>MYRYEKKGPKRGVALYSYSAEFGLTKTLEDCFEDLHDMGAHGIEILANTHIENYPYPTDEWVEKWWRLCDKYEIVPVEYGNWIDSHVLGDRDLTTEESVEMLKRDIRLAHRLGFTVMRTKMPVINDLLEPVENWKEIIKGALPLAEELGIKMCPEIHTPSNLKGKLVNDFVEFIKETGTKNFGLNIDFSVFRTSFAEGEWVDPNYTPNKPEDIIPLLPYVYCCHAKFIHMSDDFKETTIPYEEVVKTMEDNGYEGYLLSEYEGADKYDEGYEVGQTLRKHHILLKNLLGD[4x];>MEKQVIQSVGFRNIKNGNGEITGFQFKVKLPYYRGVFLSQIRPGTLFVDGQKIEKDQITWTINGEEYTNQEMRGDFKTHWATTKPAVLKVKMPGGLAQGYHDLKYGFCFTSSYMPPIIQDGLDPDKESMVYMPEFGHHVNERRLLIVKLAAALEHHHHHH[4x]

Here, we present the identification and structural basis for the activation of xenobiotic C-glycosides by heterocomplex C-deglycosylation enzymes from intestinal and soil bacteria. They are found to be metal-dependent enzymes exhibiting broad substrate specificity toward C-glycosides. DgpA catalyzes the oxidation of the glucoside moiety of puerarin to generate 3”-oxo-puerarin, in which the 3”-oxo-sugar moiety is cleaved by an unusual C-deglycosylation enzyme complex, which is an α4β4 heterooctamer of DgpB-C, to produce daidzein. For clarity, the DgpB-C and DfgA-B complexes are referred to as PuCGD and EuCGD, respectively.

Expectedly, our studies, such as co-expression, purification, and SEC-MALS analysis of DfgA and DfgB, revealed that DfgA-B formed an α4β4 heterooctamer in solution, as in the case of DgpB-C. To obtain more structural details of C-deglycosylation enzymes, and to examine the flexibility of the lid-domain and the loop regions in PuCGD and EuCGD, we also determined the structures of PuCGD and EuCGD at 2.85 and 2.54 Å resolution, respectively, using single-particle cryo-EM. The α4β4 heterooctamer structures of both enzymes were almost identical to those of the X-ray crystal structures (RMSD values 0.6 and 0.4 Å, respectively). Intriguingly, however, the densities of the lid domain in PuCGDα and the long loops in EuCGD were disordered in the cryo-EM structures. These results suggested that open-to-closed conformational changes of the lid domain occurred upon substrate binding. Although the EuCGD complex did not possess a lid domain, the disordered loop regions would play a similar role in the active site formation. In contrast, EuCGD acted on C6-glycosylated compounds 3-5, but not on C8-glycosylated compounds 1 and 2.>[2x]GPLGSPEFELGTTEILRHSMDPPTFTFNFNNEPWVRGRH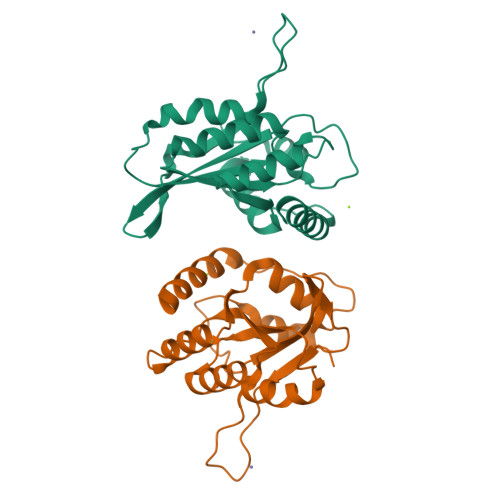ETYLCYEVERMHNDTWVKLNQRRGFLANQAPHKHGFLEGRHAELCFLDVIPFWKLDLDQDYRVTCFTSWSPCFSCAQEMAKFISKNKHVSLCIKTARIYDDQGRCQEGLRTLAEAGAKISIMTYSEFKHCWDTFVDHQGAPFQPWDGLDEHSQDLSGRLRAILQ>GSMKTIKVKNKTEGSKVAFRMLEEEITFGAKTLGLATGSTPLELYKEIRESHLDFSDMVSINLDEYVGLSADDKQSYAYFMKQNLFAAKPFKKSYLPNGLAADLAKETEYYDQILAQYPIDLQILGIGRNAHIGFNEPGT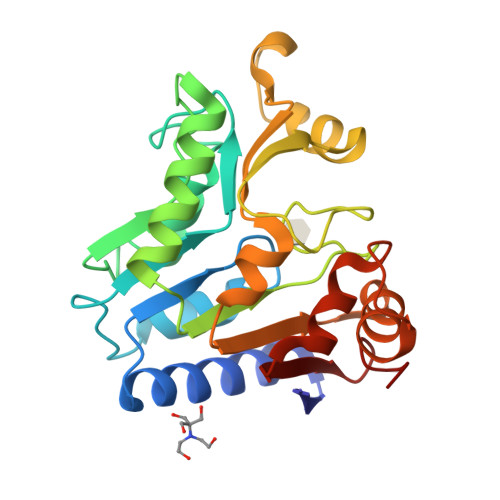AFSSQTHLVDLTPSTIAANSRFFEKAEDVPKQAISMGLASIMSAKMILLMAFGEEKAEAVAAMVKGPVTEEIPASILQTHPKVILIVDEKAGAGI[2x]>GPGSMAAATFHWDDPLLLDQQLADDERMVRDAAHAYAQGKLAPRVTEAFRHETTDAAIFREMGEIGLLGPTIPEQYGGPGLDYVSYGLIAREVERVDSGYRSMMSVQSSLVMVPIFEFGSDAQKEKYLPKLATGEWIGCFGLTEPNHGSDPGSMVTRARKVPGGYSLSGSKMWITNSPIADVFVVWAKLDEDGRDEIRGFILEKGCKGLSAPAIHGKVGLRASITGEIVLDEAFVPEENILPHVKGLRGPFTCLNSARYGIAWGALGAAESCWHIARQYVLDRKQFGRPLAANQLIQKKLADMQTEITLGLQGVLRLGRMKDEGTAAVEITSIMKRNSCGKALDIARLARDMLGGNGISDEFGVARHLVNLEVVNTYEGTHDIHALILGRAQTGIQAFF[4x]

Glutaryl-CoA dehydrogenase (GCDH) is an acyl-CoA dehydro­genase (ACDH) which catalyzes an intermediate step in the metabolic breakdown of lysine and tryptophan. Unlike other flavoproteins within this family, GCDH (EC 1.3.99.7) performs α,β-dehydrogenation as well as decarboxylation of its sub­strate glutaryl-CoA to yield the product crotonyl-CoA. Transfer of electrons from the glutaryl-CoA precursor to the electron-transfer flavoprotein is mediated by the cofactor flavin adenine dinucleotide (FAD) in both prokaryotic and eukaryotic electron-transport chains. Like other ACDHs, GCDH from B. pseudomallei (BpGCDH) exists as a homotetramer with tetrahedral symmetry and possesses an overall fold similar to that of the human enzyme.

Additional structures of BpGCDH resulting from this effort were obtained by soaking apo BpGCDH crystals in drops containing our Fragments of Life (FOL) ligand collection prior to data collection. In three of the four ligand-bound complexes fragment molecules occupy the binding site for the terminal glutamate of the glutaryl-coenzyme A substrate. The crystallographic water coordinated to the Arg97 side chain in the apo structure of BpGCDH remains in place when FOL544 is bound, but is displaced by FOL239 and FOL6421. In all three of these cases the Tyr373 side chain is rotated approximately 90° from its position in both the apo BpGCDH structure and the human ternary complex. This new position appears to facilitate ligand binding by providing a parallel aromatic surface that aligns with the heteroaromatic rings of all three fragments. Despite the presence of 100 mM HEPES in the crystallization condition and the soaking drop, neither the apo structure nor the other fragment-bound crystals of BpGCDH showed electron density for this buffer component that was sufficient for modeling. This appears to be a pH-dependent effect as FOL6421 is the only acidic fragment in the set, it is present at high concentration during the soak and no structural differences are found to account for this case. In all four fragment-bound structures Thr376 and His377 are flipped out of the α-helix observed in the apo state, partially occupying the binding pocket for the adenosine moiety of FAD. This perturbation results in a new orientation of the catalytic YEG motif. Thus, the binding of small metabolite-like ligands induces a conformation in apo crystals of BpGCDH that partially fills the FAD-binding site with protein residues.>[2x]SEGSDAPNFVLEDTNGKRIELSDLKGKGVFLNFWGTWCEPCKKEFPYMANQYKHFKSQGVEIVAVNVGESK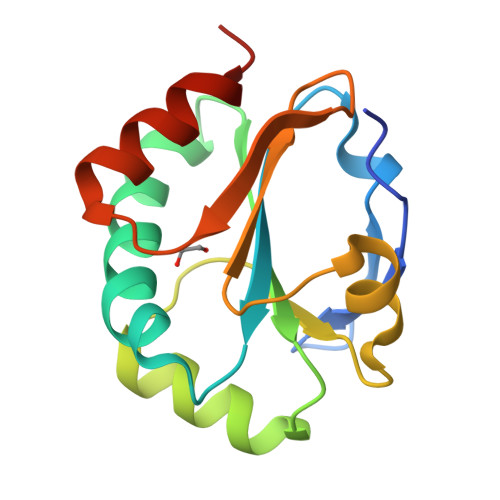IAVHNFMKSYGVNFPVVLDTDRQVLDAYDVSPLPTTFLINPEGKVVKVVTGTMTESMIHDYMNLIKPGETSG(5S)-2-amino-5-(1-ethyl-1H-pyrazol-4-yl)-3-methyl-5-[3-(pyrimidin-5-yl)phenyl]-3,5-dihydro-4H-imidazol-4-one | 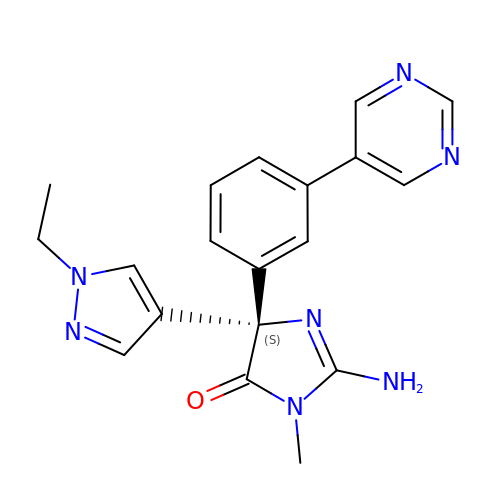C19 H19 N7 O | DNDFMOOQRXKYQL-IBGZPJMESA-N> PNFSGNWKIIRSENFEELLK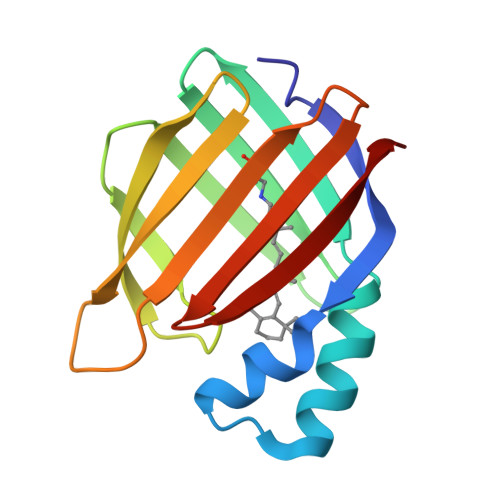VLGVNVMLRKIAVAAASKYAVEIKQEGDTFYIKVSTTVYTTEINFKVGEEFEEQTVDGRPCKSLVKWESENKMVCEQKLLKGEGPKTSWTKELTNDGELIWTMTADDVVCTQVFVRE> GPLGSPEFMAQGTLIRVTPEQPTHAVCVLGTLTQLDICSSAPEDCTSFSINASPGVVVDIAHSPPAKKKSTGSSTWPLDPGVEVTLTMKAASGSTGDQKVQISYYGPKTPPVKALLYLTAVEISLCADITRTGKVKPTRAVKDQRTWTWGPCGQGAILLVNCDRDNLESSAMDCEDDEVLDSEDLQDMSLMTLSTKTPKDFFTNHTLVLHVARSEMDKVRVFQATRGKLSSKCSVVLGPKWPSHYLMVPGGKHNMDFYVEALAFPDTDFPGLITLTISLLDTSNLELPEAVVFQDSVVFRVAPWIMTPNTQPPQEVYACSIFENEDFLKSVTTLAMKAKCKLTICPEEENMDDQWMQDEMEIGYIQAPHKTLPVVFDSPRNRGLKEFPIKRVMGPDFGYVTRGPQTGGISGLDSFGNLEVSPPVTVRGKEYP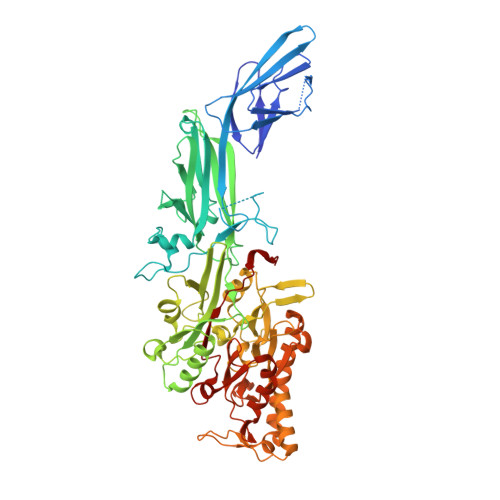LGRILFGDSCYPSNDSRQMHQALQDFLSAQQVQAPVKLYSDWLSVGHVDEFLSFVPAPDRKGFRLLLASPRSCYKLFQEQQNEGHGEALLFEGIKKKKQQKIKNILSNKTLREHNSFVERCIDWNRELLKRELGLAESDIIDIPQLFKLKEFSKAEAFFPNMVNMLVLGKHLGIPKPFGPVINGRCCLEEKVCSLLEPLGLQCTFINDFFTYHIRHGEVHAGTNVRRKPFSFKWWNMVP Methanobactins (Mbns) are a family of copper-binding peptides involved in copper uptake by methanotrophs, and are potential therapeutic agents for treating diseases characterized by disordered copper accumulation. Mbns are produced via modification of MbnA precursor peptides at cysteine residues catalyzed by the core biosynthetic machinery containing MbnB, an iron-dependent enzyme, and MbnC. Here, we present crystal structures of MbnABC complexes from two distinct species, revealing that the leader peptide of the substrate MbnA binds MbnC for recruitment of the MbnBC holoenzyme, while the core peptide of MbnA resides in the catalytic cavity created by the MbnB–MbnC interaction which harbors a unique tri-iron cluster. In both structures, the interactions between MbnA, MbnB and MbnC result in the formation of a 1:1:1 tertiary complex, and the overall structures of VcMbnABC and RrMbnABC are nearly identical.

To understand the mechanism of how MbnBCs catalyze modification of MbnAs, we finally solved the crystal structures of VcMbnABC and RrMbnABC at resolutions of 2.2 Å and 2.7 Å, respectively. In VcMbnA, the C-terminal half of the LP (residues 13–16) and the CP (residues 17–23) form a curved structure that docks into the catalytic cavity. This presents the only cysteine residue (Cys18) of VcMbnA at the apex of the curve, coordinating with one of the iron ions in the catalytic cavity formed by VcMbnBC. The divalent ion (Fe1) coordinates to VcMbnAC18 in VcMbnABC and to RrMbnAC25 in RrMbnABC, providing direct evidence for cysteine modifications of MbnA by MbnBC. In VcMbnB, the residues coordinating the iron ions are His55, His91, Glu135, Asp165, Asn168, His194, Asp209, and Glu238; this is also the case for equivalent residues in RrMbnB. Glu135 in VcMbnB provides a bidentate carboxylate ligand that bridges Fe1 and Fe2. The L2 loop of VcMbnB harbors the conserved residues Asp209 and His211, which are critical for Fe3 coordination. The main chain of VcMbnB Asp240 forms an intramolecular hydrogen bond with VcMbnBH211, while the side chain forms a hydrogen bond with the amide nitrogen of VcMbnAG19. Mutation of VcMbnBD240 to Ala, Glu or Asn had no detectable effect on VcMbnB’s interaction with VcMbnC but slightly impaired VcMbnA recognition by VcMbnBC. However, the mutation abrogated enzymatic activity of the VcMbnBC complex.

> MNVGVNWSGQRELPCINQLFLTRDIDFVELLIDNFLTTDVDSIKAFLAGRPCAFHIMNSQFLHKDERELLAMAKIINKLIHSLQPIYISDHIGKFYHRGQALPQMLEVDYGLQTHSTIKKVKAWSSLLDGKLLLENYPSIFPQDMSQIDFFKRILEETYCGLLFDISNAFIAEVNIKQSRTSWFDLIKHCQHFHIAGFENAPDNQFLVDTHSQCIEEPVLSFLQEVNNATSIATISVERDENFDVSDWALDIDNVRNRVS;> MNVGINWSGQRELPCINQLFLTRDIDFVELLIDNFLTTDVDSIKAFLAGRPCAFHIMNSQFLHKDERELLAMAKIINKLIHSLQPIYISDHIGKFYHRGQALPQMLEVDYGLQTHSTIKKVKAWSSLLDGKLLLENYPSIFPQDMSQIDFFKRILEETYCGLLFDISNAFIAEVNIKQSRTSWFDLIKHCQHFHIAGFENAPDNQFLVDTHSQCIEEPVLSFLQEVNNATSIATISVERDENFDVSDWALDIDNVRNRVS;>[2x]MEEILDRIINPLSAKPLTKKEHIYTSLVLQSSQSLILSACPSLQSQRQFCSFEYHQQFIDWCFFNKKRTDWCLALSFYQYLSYKNEQVSVEILKELIHLACSQWTYADKSTNQTVVICHTRLPSMVFGGNKSLFAQEFREVFLLETEQLKPFIQSHVPDGYFVYWILRDDSEYPSTMGEK;> MKNDKKVVVKVKDKEMTCGAFNK;> MKNDKKVVVKVKDKEMTCGAFN>MTAVSEFRPGLEGVPATLSSISFVDGQRGVLEYRGISIEQLAQQSSFLETAYLLIWGHLPTQQELTEFEHEIRYHRRIKFRIRDMMKCFPDSGHPMDALQASAAALGLFYSRRALDDPEYIRAAVVRLLAKIPTMVAAFQLIRKGNDPIQPRDELDYAANFLYMLTEREPDPVAARIFDICLTLHAEHTINASTFSAMVTASTLTDPYAVVASAVGTLAGPLHGGANEEVLDMLEAIGSVENVEPYLDHCIATKTRIMGFGHRVYKVKDPRAVILQNLAEQLFDIFGHDPYYEIAVAVEKAAAERLSHKGIYPNVDFYSGLVYRKLGIPSDLFTPVFAIARVAGWLAHWKEQLNENRIFRPTQIYTGSRNLDYTPIADRDLAIESDLEHHHHHH[54x]

Here we report the discovery of a natural protein, citrate synthase from the cyanobacterium Synechococcus elongatus, which self-assembles into Sierpiński triangles. Bacterial citrate synthase (CS) proteins are homo-oligomeric enzymes that can assemble into dimers and hexamers. CS catalyses the condensation of acetyl-CoA and oxaloacetate to citrate as the first step in the tricarboxylic acid cycle. Using cryo-electron microscopy, we reveal how the fractal assembles from a hexameric building block.

We could not obtain a structure of the 54mer from wild-type SeCS because the protein tended to aggregate on the grids. Instead, we solved this structure for a point mutant (H369R), which we generated in the course of a structure–function analysis (described further below). It produced less aggregated cryo-EM grids, which enabled us to solve a 5.9 Å structure of the 54mer. However, the dihedral angle between dimers across the interaction is different for the two types of connection within the 54mer. That is, the interaction between 6mers is made at 60°, which is identical to the angle at which it is made in a free 18mer. By contrast, the angle between 18mers within the 54mers is 34°. This different angle is necessary because the dihedral angle of interaction between hexamers is too large across the length of an 18mer to close the triangle in a 54mer.>[2x]SGAKLLQILNVRVVGSGERVVVLSHGFGTDQSAWSRVLPYLTRDHRVVLYDLVCAGSVNPDHFDFRRYDNLDAYVDDLLAILDALRIPRCAFVGHSVSAMIGILASIRRPDLFAKLVLIGASPRFLNDSDYHGGFELEEIQQVFDAMGANYSAWATGYAPLAVGADVPAAVQEFSRTLFNMRPDISLHVCQTVFKTDLRGVLGMVRAPCVVVQTTRDVSVPASVAAYLKAHLG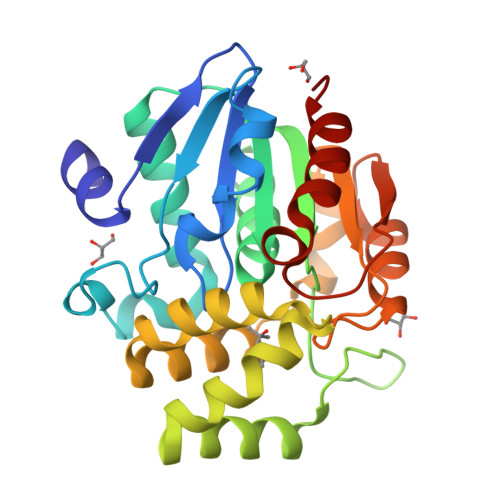GRTTVEFLQTEGHLPHLSAPSLLAQVLRRALARY> GASKIAALKEKIAALKEKIAALKEKIKDTELGMKELNEILIKEETVRRTLHNELQELRGNIRVYLRIRPALKNLENSDTSLINVNEFDDNSGVQSMEVTKIQNTAQVHEFKFDKIFDQQDTNVDVFKEVGQLVQSSLDGYNVAIFAYGQTGSGKTFTMLNPGDGIIPSTISHIFNWINKLKTKGWDYKVN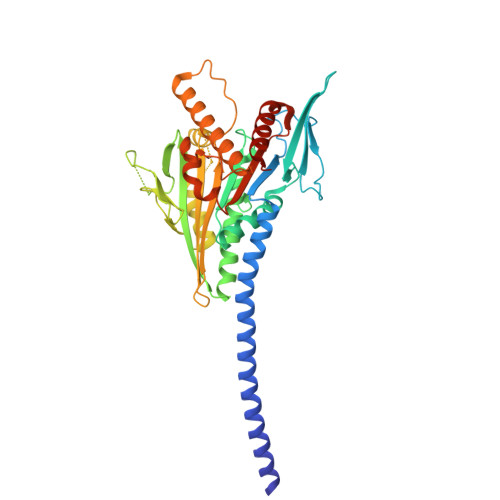AEFIEIYNENIVDLLRSDNNNKEDTSIGLKHEIRHDQETKTTTITNVTSVKLESEEMVEIILKKANKLRSTASTASNEHSSRSHSIFIIHLSGSNAKTGAHSYGTLNLVDLAGSERINVSQVVGDRLRETQNINKSLSALGDVIHALGQPDSTKRHIPFRNSKLTYLLQYSLTGDSKTLMFVNISPSSSHINETLNSLRFASKVNSTRLVSRK>[4x]SNANDLAQPIASAKVIEVELNDDYFNPNVITIPINESTTLLLKNKGKSEHTFTI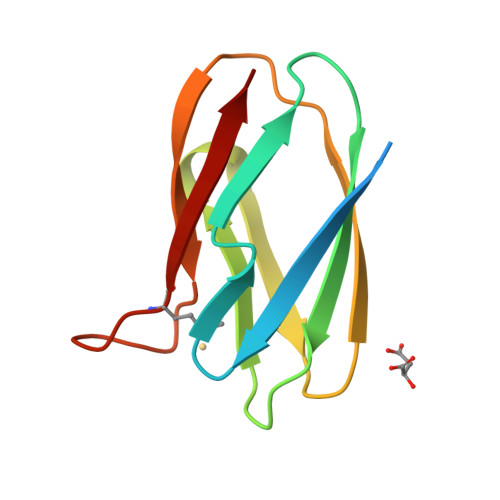KKLGIDVVVESGKEKNITVKPKSAGTYELICRYHLLKGMEGKVIVK>[2x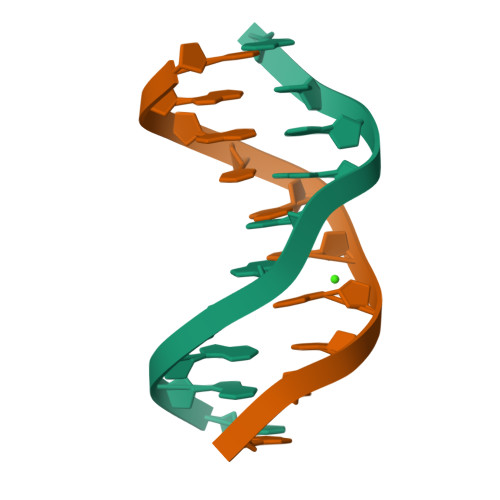]CGATATATCG> GTTKHSKLLILGSGPAGYTAAVYAARANLQPVLITGMEKGGQLTTTTEVENWPGDPNDLTGPLLMERMHEHATKFETEIIFDHINKV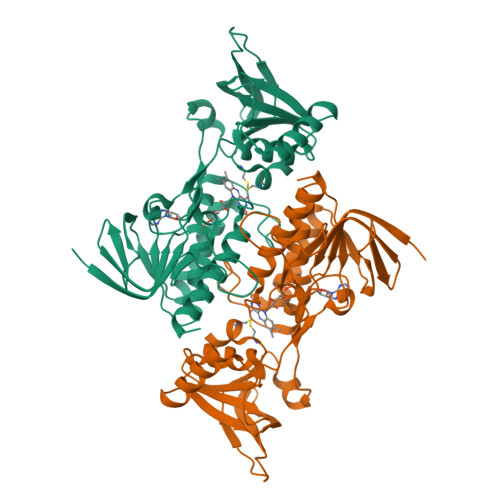DLQNRPFRLNGDNGEYTCDALIIATGASARYLGLPSEEAFKGRGVSACATCDGFFYRNQKVAVIGGGNTAVEEALYLSNIASEVHLIHRRDGFRAEKILIKRLMDKVENGNIILHTNRTLEEVTGDQMGVTGVRLRDTQNSDNIESLDVAGLFVAIGHSPNTAIFEGQLELENGYIKVQSGIHGNATQTSIPGVFAAGDVMDHIYRQAITSAGTGCMAALDAERYLDGL>[2x]MYDVTEWKHVFKLDPNKDLPDEQLEILCESGTDAVIIGGSDGVTEDNVLRMMSKVRRFLVPCVLEVSAIEAIVPGFDLYFI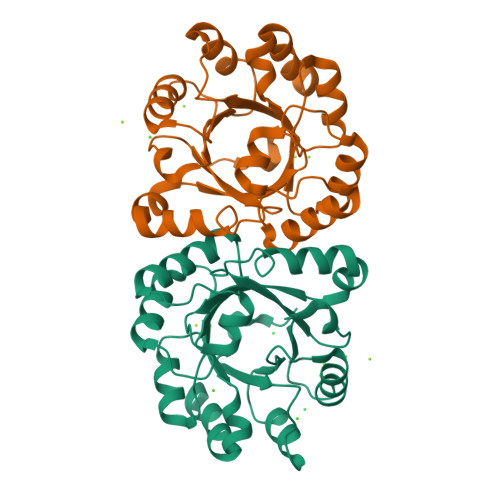PSVLNSKNADWIVGMHQKAMKEYGELMSMEEIVAEGYCIANPDCKAAALTEADADLNMDDIVAYARVSELLQLPIFYLEYSGVLGDIEAVKKTKAVLETSTLFYGGGIKDAETAKQYAEHADVIVVGNAVYEDFDRALKTVAAVKGE>MASMGTLAFDEYGRPFLIIKDQDRKSRLMGLEALKSHIMAAKAVANTMRTSLGPNGLDKMMVDKDGDVTVTNDGATILSMMDVDHQIAKLMVELSKSQDDEIGDGTTGVVVLAGALLEEAEQLLDRGIHPIRIADGYEQAARVAIEHLDKISDSVLVDIKDTEPLIQTAKTTLGSKVVNSCHRQMAEIAVNAVLTVADMERRDVDFELIKVEGKVGGRLEDTKLIKGVIVDKDFSHPQMPKKVEDAKIAILTCPFEPPKPKTKHKLDVTSVEDYKALQKYEKEKFEEMIQQIKETGANLAICQWGFDDEANHLLLQNNLPAVRWVGGPEIELIAIATGGRIVPRFSELTAEKLGFAGLVQEISFGTTKDKMLVIEQCKNSRAVTIFIRGGNKMIIEEAKRSLHDALCVIRNLIRDNRVVYGGGAAEISCALAVSQEADKCPTLEQYAMRAFADALEVIPMALSENSGMNPIQTMTEVRARQVKEMNPALGIDCLHKGTNDMKQQHVIETLIGKKQQISLATQMVRMILKIDDIRKPGESEE[4x]

TRiC interacts with approximately 10% of the entire proteome and its function is absolutely essential for viability of the cell. The general subunit architecture of the CCTs subunits comprise three distinct domains: an equatorial domain that includes the nucleotide-binding site, an apical domain involved in substrate binding, and an intermediate domain that connects the equatorial and apical domains via two hinge regions. The CCT5 homo-oligomeric complex has the two back-to-back rings of eight subunits similar to the full human TRiC complex. Moreover, the human CCT5 homo-oligomeric complex is able to hydrolyze ATP and refold misfolded protein substrates.

In this paper, we describe the crystal structure of the human CCT5 subunit. The human CCT5 and CCT5-H147R subunits were solved at 3.5 Å and 3.6 Å resolution, respectively. The CCT5 equatorial domain is formed of the N-terminal (residues 1–154) and the C-terminal (residues 418–541) regions. This domain contains two nucleotide-binding loops that interact with phosphate groups and the adenine ring of ADP. Loop-B - 103GDGTTG108 - contains the classical P-loop motif, where threonine residues coordinate the β-phosphate group of ADP. In CCT5, helix-10 consists of the residues 309EANHLLLQ316 and the proximal loop of the residues 234FSHPQMPK241. We have solved the CCT5 homo-oligomeric complex in the closed conformation, which shows intra-ring contacts between the equatorial, intermediate and apical domains. In the homo-octameric CCT5 ring, the stem loop β-strands, β1 and β2, interact with the C-terminal β-strand, β13, of an adjacent subunit. The sensor loop (also called stem-loop), 41 is located between β1 and β2 in CCT5 and it is composed of residues 63DKDGD67, where the DXXGD motif is observed for all 8 human CCT subunits. Analyzing the CCT5 sequence and the ring arrangement, the rls loop corresponds to residues 343PRFSELT349 and indeed makes contact with the substrate-binding interface from the adjacent subunit.N-[3-CHLORO-4-(4-CHLORO-2-HYDROXYPHENOXY)PHENYL]MORPHOLINE-4-CARBOXAMIDE | C17 H16 Cl2 N2 O4 | 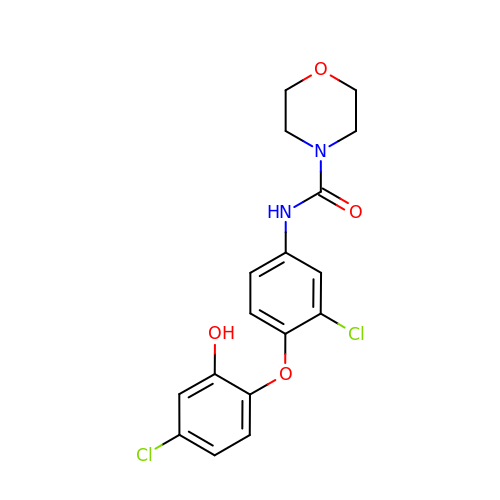SYRBFAPNWNPMEH-UHFFFAOYSA-N> MGCDAIQAAAALGEAGISSNEILELLAAAAELGLDPDAIQAAAQLGEAGISSEEIKELLRAAHELGLDPDAI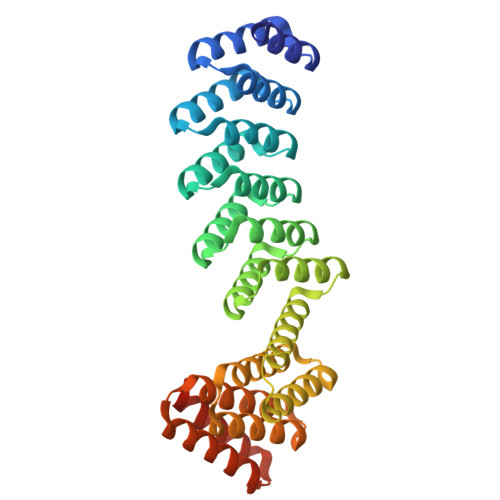AAAADLGQAGVSPVEILALLIAASVLGLDPDAIQAAAALGEAGISAEEIIELLTAARDLGLDPDAIQAAAQLGEAGISSEEIKELLRAAHELGLDPDCIAAAADLGQAGISSSEITALLLAAAAIELAKRADDKDVREIVRDALELASRSTNDEVIRLALEAAVLAARSTDSDVLEIVKDALELAKQSTNEEVIKLALKAAVLAAKSTDEEVLEEVKEALRRAKESTDEEEIKEELRKAVEEAEGGSWLEHHHHHH> PISADFSEVENAPSFLSLAENTDEVLKPYTGLEIQTIITNIVGDANPNQSRIFDQDRLRGNQYSAGGLVTQNAVSAIPFTNLIPRTIRVGNILVNSANRLQITETNVSEYYSNPIIATKLSEMISDQVKNNQFSTWRRDNTSLQGFNAFDIATINTAILPNGLSLESMLLKLSLLHSIKAMNVDAASINRSQYQVIDHNTVPTIGAPAVVGVNNSPVFGEDCGGNNPVYPFGGGTGAIAFHVTLQTVPDERKSYAIFVPPAILQATSDANEALALFALSMSEWPHALYTVTKQTTDLAGANAGQQVFIPTQSTIHIGGRRVLDLIIPRREIAPNPTTLVAANAMCMVRPQAGPDATAGAIPLAAGQLFNMNFIGAPAFEEWPLTSYLYSWAGRFDITTIRQYMGRLATMVGVKDAYWAAHELNVALSQVAPKMTTAAGGWAAQAANSAQQSDVCYSSLLTVTRSAANFPLANQPAADMRVYDTDPATWNKVALGLATAANLVPEQSMDVPFVVGDARTSFWERLQAIPMCIAWTMYYHSRGI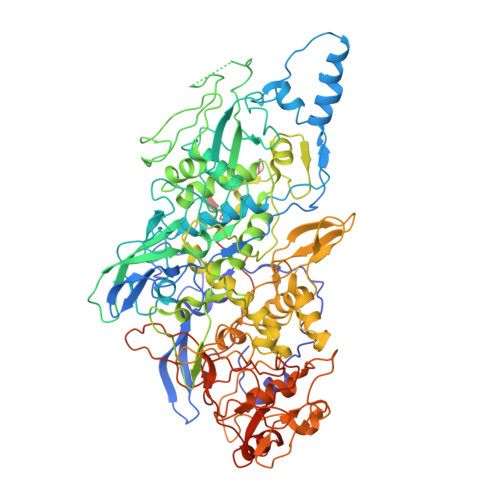TTLAWDNAYTDNTNKWLQKMVRNTFSTTQSVGTIIPARYGKIVCNLYKNMFHRAPAYVATSVGGKELHITHFERWLPGGTYANVYSGAGAVVNCFSPVLIPDIWCQYFTAKLPLFAGAFPPAQGQNSTKGFNSKQGLMIHRNQNNNLVAPYLEKFADNSSYFPVGQGPEINDMATWNGRLWMTTGNVQYLDYSGAAIVEAVPPAGELPVGKQIPLLAGENAPIELTNAATTCVPRYSNDGRRIFTYLTTAQSVIPVQACNRAANLARSCWLLSNVYAEPALQALGDEVEDAFDTLTNSSF> GSHMANLDRTDDLV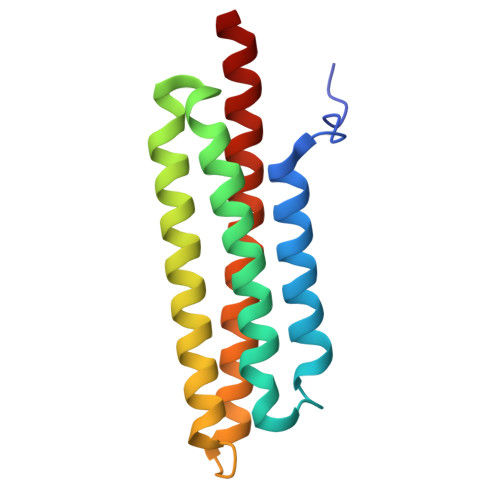YLNVMELVRAVLELKNELSQLPPEGYVVVVKNVGLTLRKLIGSVDDLLPSLPSSSRTEIEGTQKLLNKDLAELINKMRLAQQNAVTSLSEEAKRQMLTASHTLAVDAKNLLDAVDQAKVLANLAH> MRRLAFLVVAFCLAVGCFFSPVSKAEGVMSGGDGDKVAVGKDGMVATAHPLASKIGAEVLKKGGNAIDAAIAIQYALNVTEPMMSGIGGGGFMMVYDGETKETSIINSRERAPEGAKPDMFLDEDGKVIPFSERSRHGNAVGVPGTLKGLEAAHKKWGTKKMEDLISPSIKLTEEGFPIDSVLADAIKDHQDKLSKTAAKDIFLPDGEPLKEGDILVQKDMAKTFKLIRKEGSKAFYDGEIGRAIADVVQDFGGSMTPDDLSRYEVTTDKPIWGEYHGYDIASMPPPSSGGVFMLQMLKLIDDFHLSQYDPKSFEKYHLLAETMHLSYADRAAYAGDPEFVDVPLRGLLDPDYIKERQKLISLDSMNRDVKEGDPWKYEEGEPNYEIVPQPEDKTIGEATHFTVTDQWGNVVSYTTTIEQLFGTGILVPGYGLFLNNELTDFDA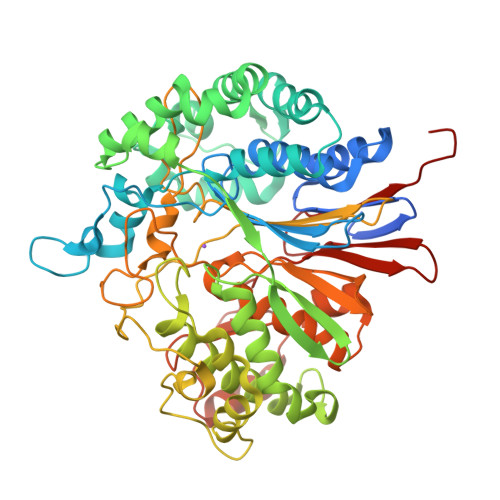IPGGANEVQPNKRPLSSMTPTIVFKDEKPVLTVGSPGGTTIIASVFQTILNYFEYGMSLQDAIEEPRIYTNSLTSYRYESGMPEDVRRKLNDFGHKFGSNPVDIGNVQSIFIDRENKTFMGVADSSRNGTAVGVNIKTSAK>[2x]AKVGFIGAGKIGQTIAYSALVSGAVDEAVIYDIIPELPDKFEHELRHAFATKGIKANVLGTNSLDDVSGMDIVVISAGKPRKPGMSRRDLFVDNAKIMIDLAQKLPSKNPGAIYLMVANPVDMMASVFMKYSKQFTISAGDQVETMRMRSFIAKKLKIPVTSVDGFVGGEHGEDAVVLWSTVKIKGKPVDE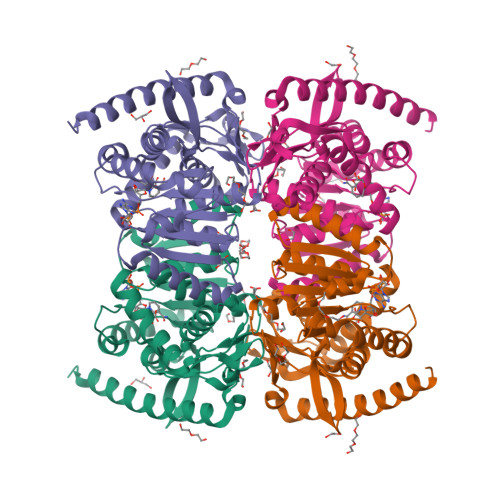FNINKDEVSDYVKKIPGEIIRVIGGTTWGPGTIIADIIKSIAFSENRVMSIATPKEYEKEIIHVSAPTVVGSSIGPSLESLLDEKDRWHLNSAMKDFYEAYKENLKQLEQAT> GSPGISGGGGGSHIEGYECQPIFLNVLEAIEPGVVCAGHDNNQPDSFAALLSSLNELGERQLVHVVKWAKALPGFRNLHVDDQMAVIQYSWMGLMVFAMGWRSFTNVNSRMLYFAPDLVFNEYRMHKSRMYSQCVRMRHLSQEFGWLQITPQEFLCMKALLLFSIIPVDGLKNQKFFDELRMNYIKELDRIIACKRKNPTSCSRRFYQLTKLLDSVQPIARELHQFTFDLLIKSHMVSVDFPEMMAEIISVQVPKILSGKVKPIYFHTQ;> SSRGLLWDLLTKDSRSGSGK

The androgen receptor (AR) is the cellular mediator of the actions of the hormone 5-α dihydrotestosterone (DHT). Androgen binding to AR leads to activation of genes involved in the development and maintenance of the male reproductive system and other tissues such as bone and muscle. AR is distinguished from other nuclear receptors in that after hormone binding, it preferentially responds to a specialized set of coactivators bearing aromatic-rich motifs, while responding poorly to coactivators bearing the leucine-rich “NR box” motifs favored by other nuclear receptors. Structures of AR in complex with FxxLF, LxxLL, FxxLW, WxxLF, WxxVW, FxxFF, and FxxYF motifs reveal a changing surface of the AR coactivator binding interface that permits accommodation of both AR-specific aromatic-rich motifs and canonical leucine-rich motifs.

The preference of AR for motifs with aromatic groups over leucine-rich motifs was assessed with a crystal structure of the AR LBD in complex with the LxxLL peptide. The LxxLL motif adopts a helical conformation, and interactions of the motif with the AF-2 cleft are predominantly hydrophobic, with the three leucine residues of the motif contributing most of the interactions. Second, the LxxLL peptide backbone forms hydrogen bonds with only one of the two conserved charge clamp residues, Lys720. A shift in the position of the LxxLL peptide helix precludes direct interactions with Glu897. This shift results from changes in the geometry of the +1 and +5 subsites mediated by Met734, which moves 2.5Å toward the +1 pocket and enables binding of a leucine at the +5 subsite by a simultaneous widening and shallowing of the pocket. Side chains of residues flanking the first leucine of the motif make additional hydrophobic interactions with the AR surface. Trp+2 reaches over Met734, clamping the methionine in between itself and Leu+1. Leu−1 extends over Met894, abutted against Glu893. These interactions likely explain the moderate affinity of AR for this particular LxxLL motif despite suboptimal complimentarity with the residues of the core motif ( ) and the loss of main chain interactions with Glu897.>[3x]SMDFRIGQGYDVHQLVPGRPLIIGGVTIPYERGLLGHSDADVLLHAITDALFGAAALGDIGRHFSDTDPRFKGADSRALLRECASRVAQAGF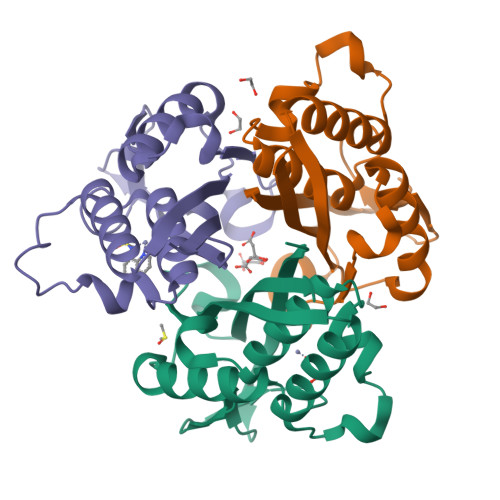AIRNVDSTIIAQAPKLAPHIDAMRANIAADLDLPLDRVNVKAKTNEKLGYLGRGEGIEAQAAALVVREAAA methyl N-(carboxymethyl)-N-(3-phenylpropyl)glycyl-L-histidinate | C20 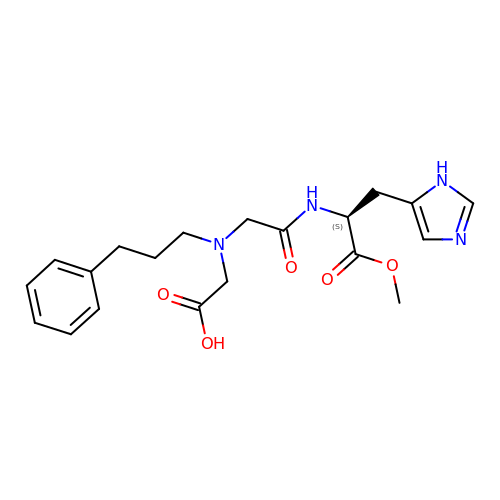H26 N4 O5 | OLFNGPVNZBLJOR-KRWDZBQOSA-N>AQCEATIESNDAMQYNLKEMVVDKSCKQFTVHLKHVGKMAKVAMGHNWVLTKEADKQGVATDGMNAGLAQDYVKAGDTRVIAHTKVIGGGESDSVTFDVSKLTPGEAYAYFCSFPGHWAMQKGTLKLSN[2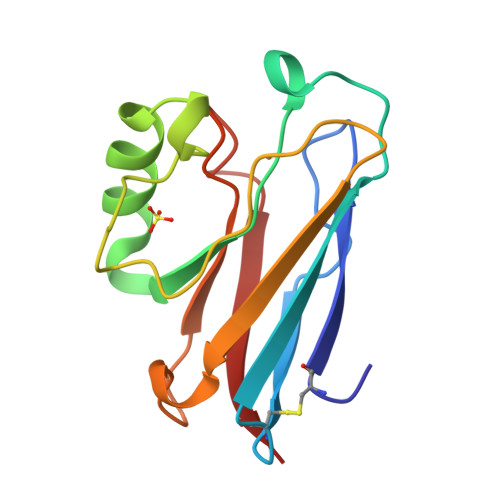x]> LEEKKVCQGTSNKLTQLGTFEDHFLSLQRMFNNCEVVLGNLEITYVQRNYDLSFLKTIQEVAGYVLIALNTVERIPLENLQIIRGNMYYENSYALAVLSNYDANKTGLKELPMRNLQEILHGAVRFSNNPALCNVESIQWRD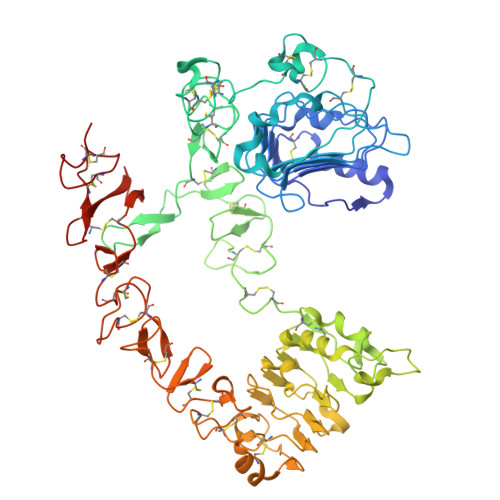IVSSDFLSNMSMDFQNHLGSCQKCDPSCPNGSCWGAGEENCQKLTKIICAQQCSGRCRGKSPSDCCHNQCAAGCTGPRESDCLVCRKFRDEATCKDTCPPLMLYNPTTYQMDVNPEGKYSFGATCVKKCPRNYVVTDHGSCVRACGADSYEMEEDGVRKCKKCEGPCRKVCNGIGIGEFKDSLSINATNIKHFKNCTSISGDLHILPVAFRGDSFTHTPPLDPQELDILKTVKEITGFLLIQAWPENRTDLHAFENLEIIRGRTKQHGQFSLAVVSLNITSLGLRSLKEISDGDVIISGNKNLCYANTINWKKLFGTSGQKTKIISNRGENSCKATGQVCHALCSPEGCWGPEPRDCVSCRNVSRGRECVDKCKLLEGEPREFVENSECIQCHPECLPQAMNITCTGRGPDNCIQCAHYIDGPHCVKTCPAGVMGENNTLVWKYADAGHVCHLCHPNCTYGCTGPGLEGCPTNGPKHHHHHH>[4x]MYLTKEEELILAGEYGYALQKAMEILVALGDIYGADRLIPIKSAQVAGVSYKNIGDAGIEFLRDFVEAGAKVSVYTTLNPAGIGDDEFMEKQMEVLELYRKMGIEVTSTCTPYYGANLPKFGDHIAWSESSAVSFANSILGARTNREGGPSSLAAAIVGKTPNYGLHLDENRKATVIVDVKAKVKTFADYSVLGYHVGKTLGNDVPYFKNLKPEKTEFLKELGAAMGATGSIA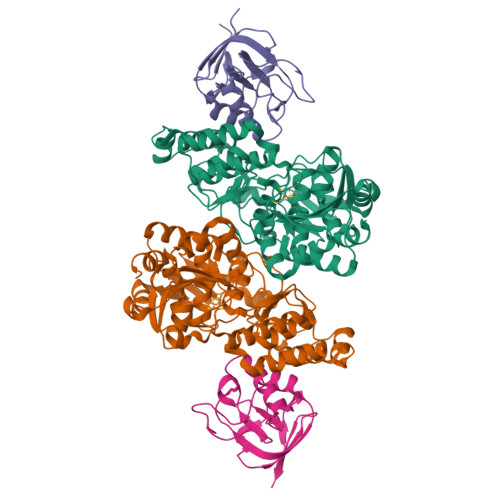LYHVEGETPEYREAITDKLETITVEDSDLKAVRESFQDDWSDIDMILIGCPHASLPEVKEIAELLRMRGKPLKIPLFITASRAVKALADALGYTEIIERYNGKIIPDSCFVVSPIKGWYRGIATNSGKSAFYFRSFGFSVRLDDVENLIKEAP;>[4x]GPKLKGRKIVGGKAEGEVIVSRKPLSFLGGVDPETGIVTDAESDIRGQSIAGKILVFPRGKGSTVGSYVIYALKKNNKAPKAIIVGEAETIVATGAIISDIPMVDGVDVSKLKTGMKVRVDADSGEVEILEDGE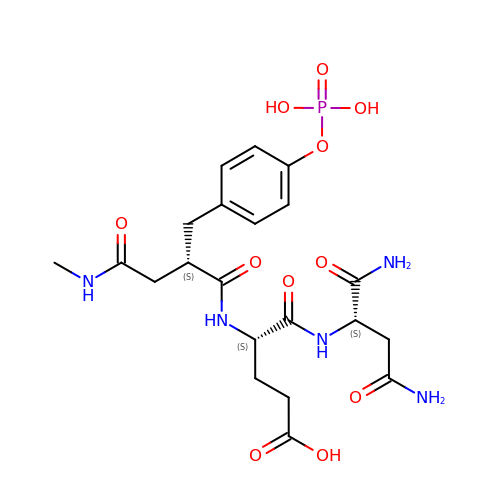N-{(2S)-4-(methylamino)-4-oxo-2-[4-(phosphonooxy)benzyl]butanoyl}-L-alpha-glutamyl-L-aspartamide | C21 H30 N5 O11 P | NPYWTYXAKSZNLF-QEJZJMRPSA-N> MENAHTKTVEEVLGHFGVNESTGLSLEQVKKLKERWGSNELPAEEGKTLLELVIEQFEDLLVRILLLAACISFVLAWFEEGEETITAFVEPFVILLILVANAIVGVWQERNAENAIEALKEYEPEMGKVYRQDRKSVQRIKAKDIVPGDIVEIAVGDKVPADIRLTSIKSTTLRVDQSILTGESVSVIKHTDPVPDPRAVNQDKKNMLFSGTNIAAGKAMGVVVATGVNTEIGKIRDEMVATEQERTPLQQKLDEFGEQLSKVISLICIAVWIINIGHFNDPVHGGSWIRGAIYYFKIAVALAVAAIPEGLPAVITTCLALGTRRMAKKNAIVRSLPSVETLGCTSVICSDKTGTLTTNQMSVCRMFILDKVEGDTCSLNEFTITGSTYAPIGEVHKDDKPVKCHQYDGLVELATICALCNDSALDYNEAKGVYEKVGEATETALTCLVEKMNVFDTELKGLSKIERANACNSVIKQLMKKEFTLEFSRDRKSMSVYCTPNKPSRTSMSKMFVKGAPEGVIDRCTHIRVGSTKVPMTPGVKQKIMSVIREWGSGSDTLRCLALATHDNPMRREEMNLEDSANFIKYETNLTFVGCVGMLDPPRIEVASSVKLCRQAGIRVIMITGDNKGTAVAICRRIGIFGQDEDVTSKAFTGREFDELNPSAQREACLNARCFARVEPSHKSKIVEFLQSFDEITAMTGDGVNDAPALKKSEIGIAMGSGTAVAKTASEMVLADDNFSTIVAAVEEGRAIYNNMKQFIRYLISSNVGEVVCIFLTAALGFPEALIPVQLLWVNLVTDGLPATALGFNPPDLDIMNKPPRNPKEPLISGWLFFRYLAIGCYVGAATVGAAAWWFIAADGGPRVTFYQLSHFLQCKEDNPDFEGVDCAVFESPYPMTMALSVLVTIEMCNALNSLS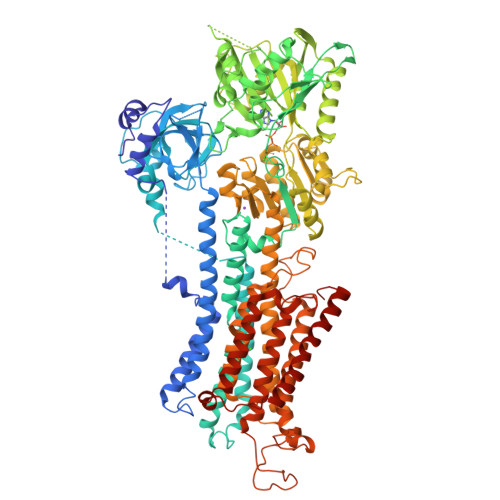ENQSLLRMPPWENIWLVGSICLSMSLHFLILYVEPLPLIFQITPLNLTQWLMVLKISLPVILMDETLKFVARNYLEPAILE>[2x]SMGVTVQDICFAFLQNYYERMRTDPSKLAYFYASTAELTHTNYQSKSTNEKDDVLPTVKVTGRENINKFFSRNDAKVRSLKLKLDTIDFQYTGHLHKSILIMATGEMFWTGTPV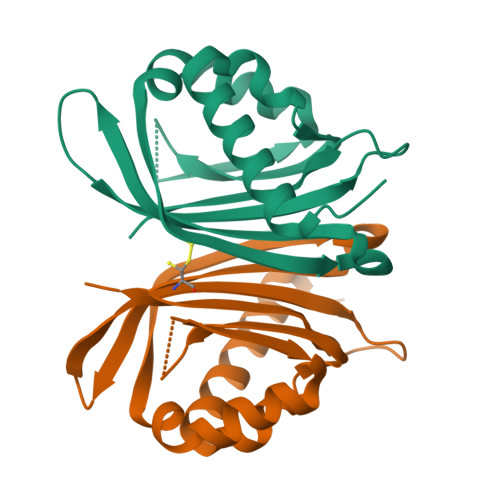YKFCQTFILLPSSNGSTFDITNDIIRFISNSFK> DPFTHMSDKIDEMYDIFGD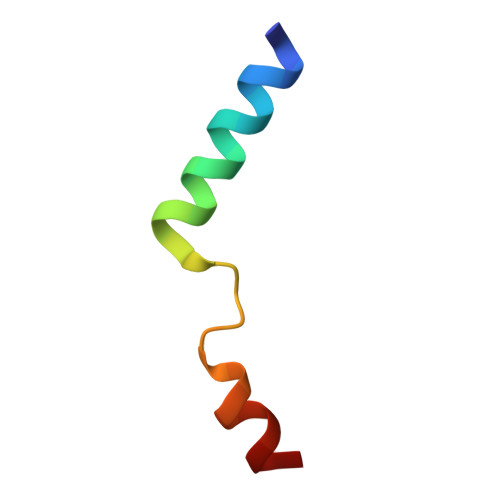GHDYDWALEIEN>[3x]GS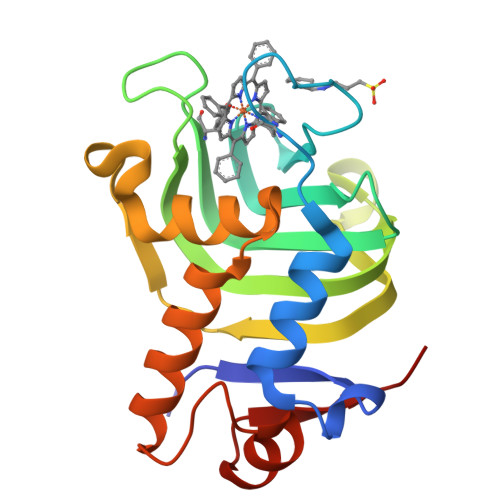MSISISYSTTYSGWTVADYLADWSAYFGDVNHRPGQVVDGSNTGGFNPGPFDGSQYALKSTASDAAFIAGGDLHYTLFSNPSHTLWGKLDSIALGDTLTGGASSGGYALDSQEVSFSNLGLDSPIAQGRDGTVHKVVYGLMSGDSSALQGQIDALLKAVDPSLSINSTFDQLAAAGVAHATPAA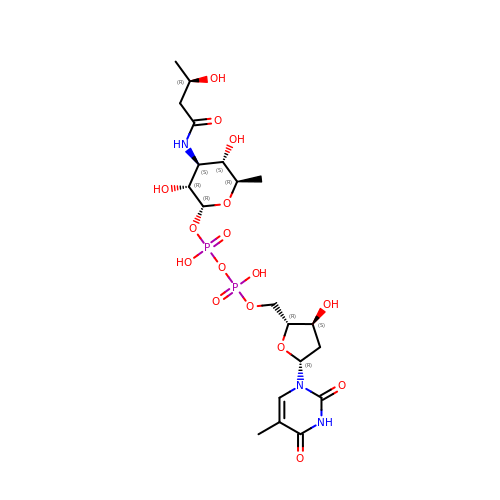[[(2~{R},3~{S},5~{R})-5-[5-methyl-2,4-bis(oxidanylidene)pyrimidin-1-yl]-3-oxidanyl-oxolan-2-yl]methoxy-oxidanyl-phosphoryl] [(2~{R},3~{R},4~{S},5~{S},6~{R})-6-methyl-3,5-bis(oxidanyl)-4-[[(3~{R})-3-oxidanylbutanoyl]amino]oxan-2-yl] hydrogen phosphate | C20 H33 N3 O16 P2 | SFDGKYQEVYNQBU-VTFQMSFESA-N>[6x]MSELKLKPLPKVELPPDFVDVIRIKLQGKTVRTGDVIGISILGKEVKFKVVQAYPSPLRVEDRTKI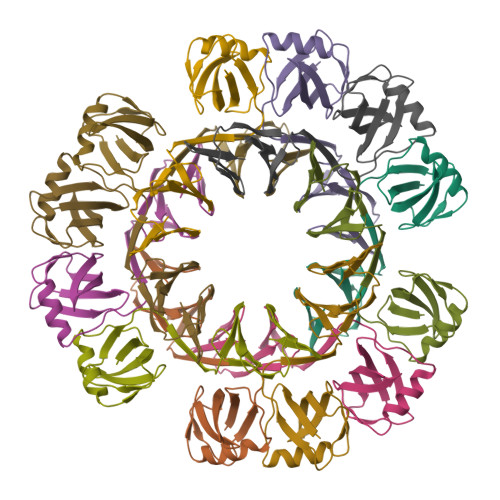TLVTHPVDVLEAKIKGIKDVILDENLIVVITEENEVLIFNQNLEELYRGKFENLNKVLVRNDLVVIIDEQKLTLIRT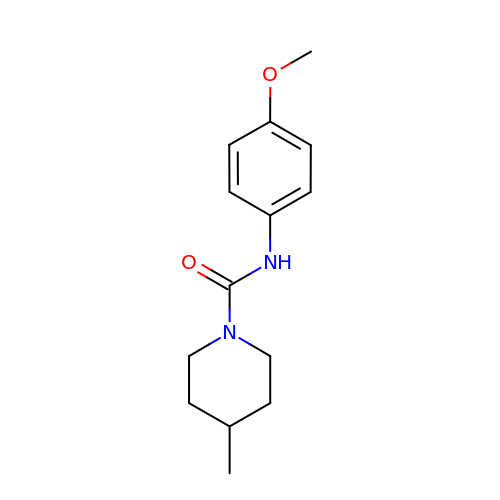~{N}-(4-methoxyphenyl)-4-methyl-piperidine-1-carboxamide | C14 H20 N2 O2 | YJMGSVPGOIBYHC-UHFFFAOYSA-N>GGMILLIDNYDSFTWNLYQYFCELGADVLVKRNDALTLADIDALKPQKIVISPGPCTPDEAGISLDVIRHYAGRLPILGVCLGHQAMAQAFGGKVVRAAKVMHGKTSPITHNGEGVFRGLANPLTVTRYHSLVVEPDSLPACFDVTAWSETREIMGIRHRQWDLEGVQFHPESILSEQGHQLLANFLHR[2x];>[2x]HMKTLSPAVITLLWRQDAAEFYFSRLSHLPWAMLLHSGYADHPYSRFDIVVAEPICTLTTFGKETVVSESEKRTTTTDDPLQVLQQVLDRADIRPTHNEDLPFQGGALGLFGYDLGRRFESLPEIAEQDIVLPDMAVGIYDWALIVDHQRHTVSLLSHNDVNARRAWLESQQFSPQEDFTLTSDWQSNMTREQYGEKFRQVQEYLHSGDCYQVNLAQRFHATYSGDEWQAFLQLNQANRAPFSAFLRLEQGAILSLSPERFILCDNSEIQTRPIKGTLPRLPDPQEDSKQAVKLANSAKDRAENLMIVDLMRNDIGRVAVAGSVKVPELFVVEPFPAVHHLVSTITAQLPEQLHASDLLRAAFPGGSITGAPKVRAMEIIDELEPQRRNAWCGSIGYLSFCGNMDTSITIRTLTAINGQIFCSAGGGIVADSQEEAEYQETFDKVNRILKQLEK

Here, we chose aminodeoxychorismate synthase (ADCS) from Escherichia coli, which consists of a class I glutaminase subunit (PabA) and a synthase subunit (PabB), to investigate the mechanism of glutaminase catalysis regulation and its impact on overall GAT activity. PabB catalyzes the amination of chorismate (Cho) to 4-amino-4-deoxy-chorismate, which is a committed step in folic acid biosynthesis. GATs comprise minimally a glutaminase that produces ammonia, which reacts with a synthase-bound substrate to yield specific nitrogen-containing products. As evidenced by analytical gel filtration and isothermal titration calorimetry (ITC) data, the PabA and PabB subunits form a heterodimeric assembly with a dissociation constant KD = 0.16 ± 0.06 μM.

When the crystallization buffer was incubated with EDTA, in the resulting X-ray structure, the density assigned to Zn2+ also disappeared. Comparison of the glutaminase active site geometry in the presence and absence of Zn2+ allowed to identify conformational changes associated with Zn2+ binding. While we did not detect any significant positional changes for the catalytic triad residues aC79, aH168, and aE170, the side chain of aH128 flips from an orientation blocking the PabA active site in the presence of Zn2+ to a conformation, in which it integrates into an interaction network forming the glutaminase active site in a catalytically competent conformation, in the absence of Zn2+. Finally, in all ADCS complex structures without Zn2+, we found a second well-defined and structurally conserved water molecule in the glutaminase active site. It is located approximately midway between the imidazole side-chain groups of aH128 and aH168, suggesting that it critically contributes to the establishment of a catalytically competent conformation of the ADCS glutaminase active site. The associated changes are most visibly illustrated by a long-range movement of residue bE119 from the PabB subunit, which is 10−13 Å from any PabA residues in different ADCS structures devoid of Gln-TE in the glutaminase active site.>GAMAPVPVTKLVCDGDTYKCTAYLDFG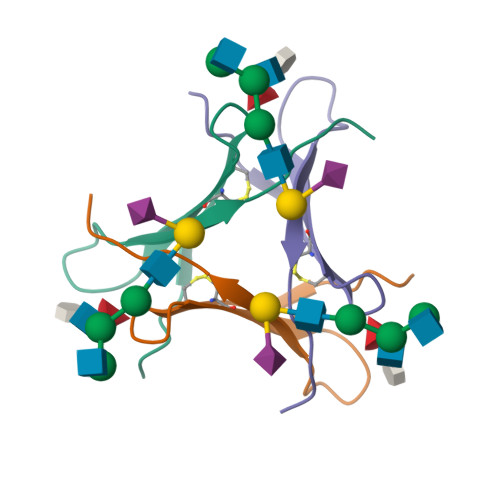DGRWVAQWDTNVFHTG[2x]>[2x]MEMDYKDDDDKGGGGGASTMSGTKPDILWAPHHVDRFVVCDSELSLYHVESTVNSELKAGSLRLSEDSAATLLSINSDTPYMKCVAWYLNYDPECLLAVGQANGRVVLTSLGQDHNSKFKDLIGKEFVPKHARQCNTLAWNPLDSNWLAAGLDKHRADFSVLIWDICSKYTPDIVPMEKVKLSAGETETTLLVTKPLYELGQNDACLSLCWLPRDQKLLLAGMHRNLAIFDLRNTSQKMFVNTKAVQGVTVDPYFHDRVASFYEGQVAIWDLRKFEKPVLTLTEQPKPLTKVAWCPTRTGLLATLTRDSNIIRLYDMQHTPTPIGDETEPTIIERSVQPCDNYIASFAWHPTSQNRMIVVTPNRTMSDFTVFERISLAWSPITSLMWACGRHLYECTEEENDNSLEKDIATKMRLRALSRYGLDTEQVWRNHILAGNEDPQLKSLWYTLHFMKQYTEDMDQKSPGNKGSLVYAGIKSIVKSSLGMVESSRHNWSGLDKQSDIQNLNEERILALQLCGWIKKGTDVDVGPFLNSLVQEGEWERAAAVALFNLDIRRAIQILNEGASSEKGDLNLNVVAMALSGYTDEKNSLWREMCSTLRLQLNNPYLCVMFAFLTSETGSYDGVLYENKVAVRDRVAFACKFLSDTQLNRYIEKLTNEMKEAGNLEGILLTGLTKDGVDLMESYVDRTGDVQTASYCMLQGSPLDVLKDERVQYWIENYRNLLDAWRFWHKRAEFDIHRSKLDPSSKPLAQVFVSCNFCGKSISYSCSAVPHQGRGFSQYGVSGSPTKSKVTSCPGCRKPLPRCALCLINMGTPVSSCPGGTKSDEKVDLSKDKKLAQFNNWFTWCHNCRHGGHAGHMLSWFRDHAECPVSACTCKCMQLDTTGNLVPAETVQP;> MEKMSRVTTALGGSVLTGRTMHCHLDAPANAISVCRDAAQVVVAGRSIFKIYAIEEEQFVEKLNLRVGRKPSLNLSCADVVWHQMDENLLATAATNGVVVTWNLGRPSRNKQDQLFTEHKRTVNKVCFHPTEAHVLLSGSQDGFMKCFDLRRKDSVSTFSGQSESVRDVQFSIRDYFTFASTFENGNVQLWDIRRPDRCERMFTAHNGPVFCCDWHPEDRGWLATGGRDKMVKVWDMTTHRAKEMHCVQTIASVARVKWRPECRHHLATCSMMVDHNIYVWDVRRPFVPAAMFEEHRDVTTGIAWRHPHDPSFLLSGSKDSSLCQHLFRDASQPVERANPEGLCYGLFGDLAFAAKESLVAAESGRKPYTGDRRHPIFFKRKLDPAEPFAGLASSALSVFETEPGGGGMRWFVDTAERYALAGRPLAELCDHNAKVARELGRNQVAQTWTMLRIIYCSPGLVPTANLNHSVGKGGSCGLPLMNSFNLKDMAPGLGSETRLDRSKGDARSDTVLLDSSATLITNEDNEETEGSDVPADYLLGDVEGEEDELYLLDPEHAHPEDPECVLPQEAFPLRHEIVDTPPGPEHLQDKADSPHVSGSEADVASLAPVDSSFSLLSVSHALYDSRLPPDFFGVLVRDMLHFYAEQGDVQMAVSVLIVLGERVRKDIDEQTQEHWYTSYIDLLQRFRLWNVSNEVVKLSTSRAVSCLNQASTTLHVNCSHCKRPMSSRGWVCDRCHRCASMCAVCHHVVKGLFVWCQGCSHGGHLQHIMKWLEGSSHCPAGCGHLCEYS;> MAARWSSENVVVEFRDSQATAMSVDCLGQHAVLSGRRFLYIVNLDAPFEGHRKISRQSKWDIGAVQWNPHDSFAHYFAASSNQRVDLYKWKDGSGEVGTTLQGHTRVISDLDWAVFEPDLLVTSSVDTYIYIWDIKDTRKPTVALSAVAGASQVKWNKKNANCLATSHDGDVRIWDKRKPSTAVEYLAAHLSKIHGLDWHPDSEHILATSSQDNSVKFWDYRQPRKYLNILPCQVPVWKARYTPFSNGLVTVMVPQLRRENSLLLWNVFDLNTPVHTFVGHDDVVLEFQWRKQKEGSKD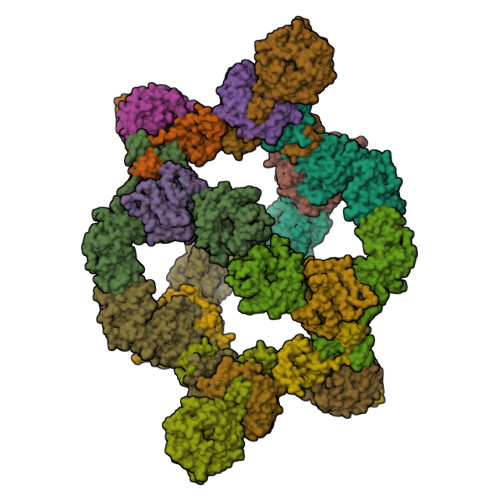YQLVTWSRDQTLRMWRVDSQMQRLCANDILDGVDEFIESISLLPEPEKTLHTEDTDHQHTASHGEEEALKEDPPRNLLEERKSDQLGLPQTLQQEFSLINVQIRNVNVEMDAADRSCTVSVHCSNHRVKMLVKFPAQYPNNAAPSFQFINPTTITSTMKAKLLKILKDTALQKVKRGQSCLEPCLRQLVSCLESFVNQEDSASSNPFALPNSVTPPLPTFARVTTAYGSYQDANIPFPRTSGARFCGAGYLVYFTRPMTMHRAVSPTEPTPRSLSALSAYHTGLIAPMKIRTEAPGNLRLYSGSPTRSEKEQVSISSFYYKERKSRRWKSKREGSDSGNRQIKAAGKVIIQDIACLLPVHKSLGELYILNVNDIQETCQKNAASALLVGRKDLVQVWSLATVATDLCLGPKSDPDLETPWARHPFGRQLLESLLAHYCRLRDVQTLAMLCSVFEAQSRPQGLPNPFGPFPNRSSNLVVSHSRYPSFTSSGSCSSMSDPGLNTGGWNIAGREAEHLSSPWGESSPEELRFGSLTYSDPRERERDQHDKNKRLLDPANTQQFDDFKKCYGEILYRWGLREKRAEVLKFVSCPPDPHKGIEFGVYCSHCRSEVRGTQCAICKGFTFQCAICHVAVRGSSNFCLTCGHGGHTSHMMEWFRTQEVCPTGCGCHCLLESTF;>MFVARSIAADHKDLIHDVSFDFHGRRMATCSSDQSVKVWDKSESGDWHCTASWKTHSGSVWRVTWAHPEFGQVLASCSFDRTAAVWEEIVGESNDKLRGQSHWVKRTTLVDSRTSVTDVKFAPKHMGLMLATCSADGIVRIYEAPDVMNLSQWSLQHEISCKLSCSCISWNPSSSRAHSPMIAVGSDDSSPNAMAKVQIFEYNENTRKYAKAETLMTVTDPVHDIAFAPNLGRSFHILAIATKDVRIFTLKPVRKELTSSGGPTKFEIHIVAQFDNHNSQVWRVSWNITGTVLASSGDDGCVRLWKANYMDNWKCTGILKGNGSPVNGSSQQGTSNPSLGSTIPSLQNSLNGSSAGRYFFTPLDSPRAGSRWSSYAQLLPPPPPPLVEHSCDADTANLQYPHPRRRYLSRPLNPLPENEGI[3x];> MVSVINTVDTSHEDMIHDAQMDYYGTRLATCSSDRSVKIFDVRNGGQILIADLRGHEGPVWQVAWAHPMYGNILASCSYDRKVIIWREENGTWEKSHEHAGHDSSVNSVCWAPHDYGLILACGSSDGAISLLTYTGEGQWEVKKINNAHTIGCNAVSWAPAVVPGSLIDHPSGQKPNYIKRFASGGCDNLIKLWKEEEDGQWKEEQKLEAHSDWVRDVAWAPSIGLPTSTIASCSQDGRVFIWTCDDASSNTWSPKLLHKFNDVVWHVSWSITANILAVSGGDNKVTLWKESVDGQWVCISDVNKGQGSVSASVTEGQQNEQ>[8x]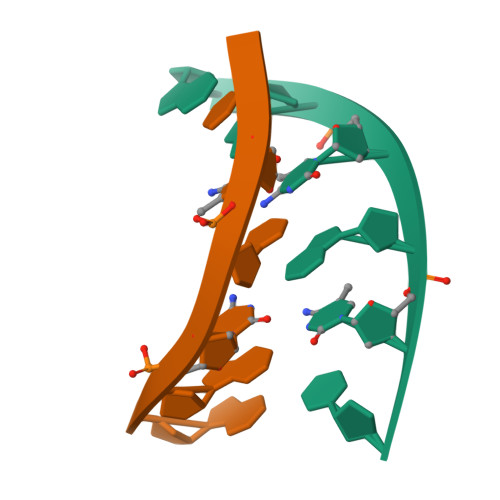GGCGCC>[2x]MQFPQLDPATLAAFSAAFRGELIWPSDADYDEARRIWNGTIDRRPALIARCTSTPDVVAAVSFARKSGLLVAVRGGGHSMAGHSVCDGGIVIDLSLMNSIKVSRRLRRARAQGGCLLGAFDTATQAHMLATPAGVVSHTGLGGLVLGGG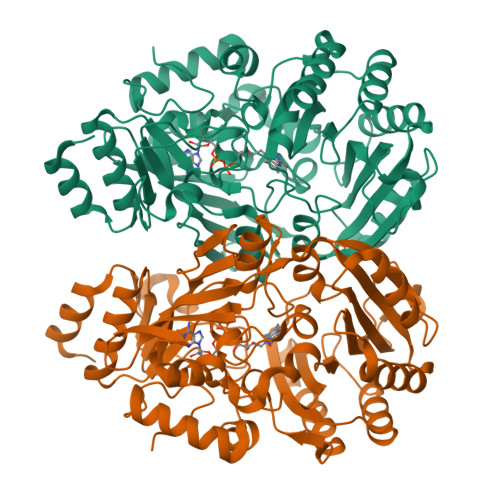FGWLSRKYGLSIDNLTSVEIVTADGGVLTASDTENPDLFWAVRGGGGNFGVVTAFEFDLHRVGPVRFASTYYSLDEGPQVIRAWRDHMATAPDELTWALYLRLAPPLPELPADMHGKPVICAMSCWIGDPHEGERQLESILHAGKPHGLTKATLPYRALQAYSFPGAVVPDRIYTKSGYLNELSDEATDTVLEHAADIASPFTQLELLYLGGAVARVPDDATAYPNRQSPFVTNLAAAWMDPTEDARHTAWAREGYRALAGHLSGGYVNFMNPGEADRTREAYGAAKFERLQGVKAKYDPTNLFRLNQNIPPSSP Brugia malayi venom allergen-like protein 1 (BmVAL-1) protein was discovered as a highly expressed transcript representing ∼2% of cDNAs from the mosquito-borne infective larval (L3) stage, and at lower levels in subsequent post-infective mammalian stages. BmVAL-1 belongs to the eukaryotic CAP (cysteine-rich secretory protein/antigen 5/pathogenesis related-1) or SCP/TAPS (Sperm-coating protein/Tpx/antigen 5/pathogenesis related-1/Sc7) superfamily of proteins, which has been implicated in biological processes such as reproduction, fungal virulence, cellular defense, and immune evasion (Hawdon et al., 1999, Ding et al., 2000, Gao et al., 2001, Zhan et al., 2003, Schneiter and Di Pietro, 2013). Immunologically, BmVAL-1 is a major target of host immunity with >90% of infected B. malayi microfilaraemic cases being seropositive for the recombinant protein, and evidence from mouse models that the antigen induces a strong T cell response. Similar to VAL proteins from other filarial parasites, BmVAL-1 has a single ∼15 kDa CAP domain.

Recombinant BmVAL-1 was produced as a glycosylated protein using a plant expression system. All 206 amino acid residues have ordered main and side chain electron density maps, of which 36 (17.5%) fold as beta strands, 59 (28.6%) fold as alpha helices, 11 (5.3%) fold as 3–10 helices, while 100 (48.5%) form loops. The overall topology of BmVAL-1 is an alpha-beta-alpha sandwich, in which a mixed strand beta sheet is sandwiched between two helical/loop regions. There are five disulfide bridges in the BmVAL-1 structure (19–69, 82–170, 164–180, 200–211 and 206–218). The last two disulfides stabilize a unique carboxyl terminus extension that is made mostly of loops. The two predicted N-linked glycosylation sites of BmVAL-1 (N52 and N138) are glycosylated and the branches have highly ordered 2Fo-Fc electron density contoured at 1.5 sigma. Some N-glycans with one terminal GlcNAc residue (MGnXF3 or GnMXF3) were also detected. The glycosylation site at N138 is within the caveolin-binding motif (CBM) loop that is required for sterol export. The overall structure of BmVAL-1 is a prototypical CRISP-type SCP/TAPS protein that has two histidine residues which coordinate divalent cations located in the large central cavity. The central cavity of BmVAL-1 has a volume of 2567 Å3 which is larger than other single CAP-domain SCP/TAPS protein structures including Na-ASP-2 (1824 Å3), Pry1CAP (1591 Å3), GLIPR-1 (2000 Å3), GAPR-1 (1303 Å3), ves v5 (2048 Å3) and tablysin-15 (2263 Å3) as assessed by PDBsum (Henriksen et al., 2001, Serrano et al., 2004, Asojo et al., 2005, Asojo et al., 2011, Ma et al., 2011, de Beer et al., 2014, Darwiche et al., 2016, Laskowski et al., 2018).

> FECPGGRLTPQQRKDIVRQNNKFRSLLIHGKLKNRNGTYMPRGKNMLLLKWSCQLENSAQRWANQCVFGHSPRNQRQGIGENVYAYWSSESVEKLRNTAGTEAGKSWWSELPKLYKQNPSNNLTDDVARQGVLHFTQMAWGKTHKIGCGIATNCDGGRTLIAICHYSPAGNMLKELIYELGEPCKTDSDCNTKKCAKKSGLCRKEL> GSPGIRLGSSEDNFARFVCKNNGVLFENQLLQIGLKSEFRQNLGRMFIFYGNKTSTQFLNFTPT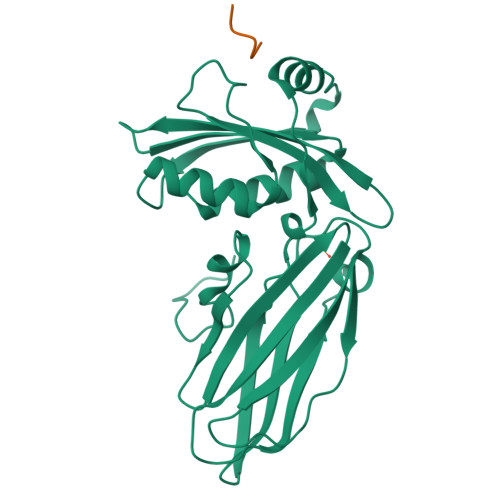LICADDLQTNLNLQTKPVDPTVDGGAQVQQVVNIECISDFTEAPVLNIQFRYGGTFQNVSVKLPITLNKFFQPTEMASQDFFQRWKQLSNPQQEVQNIFKAKHPMDTEITKAKIIGFGSALLEEVDPNPANFVGAGIIHTKTTQIGCLLRLEPNLQAQMYRLTLRTSKDTVSQRLCELLSEQF;> GSDPWK> GSMEIRVRVEKDPELGFSISG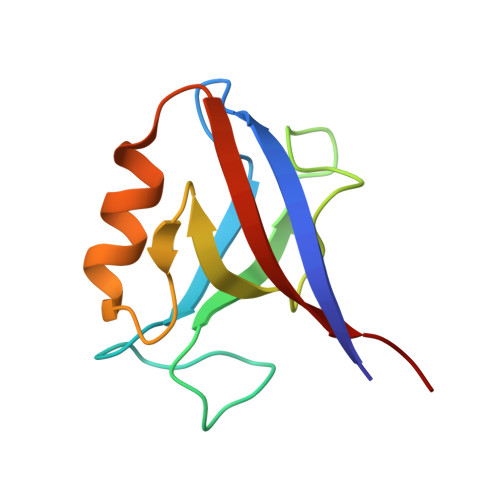GVGGRGNPFRPDDDGIFVTRVQPEGPASKLLQPGDKIIQANGYSFINIEHGQAVSLLKTFQNTVELIIVREVSS>[2x]MPLTPNDIHNKTF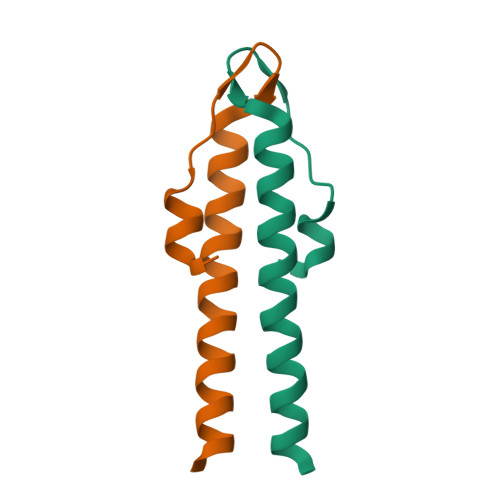TKSFRGYDEDEVNEFLAQVRKDYEIVLRKKTELEAKVNELDERI> GSSAAPGAIQCMNRHKMERHGKMPAGYKGFDCNVCDQPMLKITEKAYMYRCEKCDYDVCNQC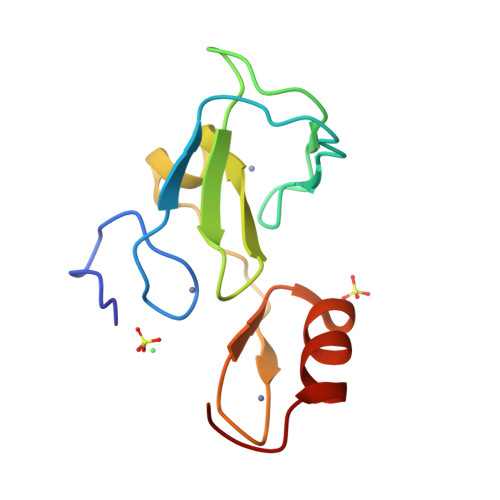AESRKFKEVHFLCAKCGKKFPSQTKLQYHSRGCRGPS> MRCIGISNRDFVEGVSGGSWVDIVLEHGSCVTTMAKNKPTLDFELIKTEAKQPATLRKYCIEAKLTNTTTESRCPTQGEPSLNEEQDKRFVCKHSMVDRGWGNGCGLFGKGGIVTCAMFRCKKNMEGKVVQPENLEYTVVITPHSGEEHAVGNDTGKHGKEVKITPQSSITEAELTGYGTVTMECSPRTGLDFNEMVLLQMENKAWLVHRQWFLDLPLPWLPGADTQGSNWIQKETLVTFKNPHAKKQDVVVLGSQEGAMHTALTGATEIQMSSGNLLFTGHLKCRLRMDKLQLKGMSYSMCTGKFKVVKEIAETQHGTIVIRVQYEGDGSPCKIPFEIMDLEKRHVLGRLITVNPIVTEKDSPVNIEA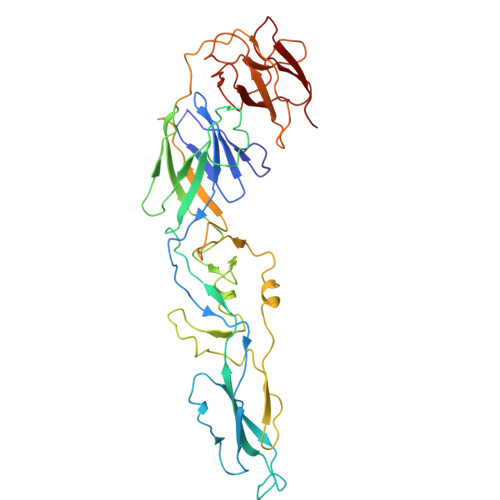EPPFGDSYIIIGVEPGQLKLDWFKKG2'-[2-(1,3-benzodioxol-5-yl)pyrimidin-4-yl]-5',6'-dihydrospiro[piperidine-4,7'-pyrrolo[3,2-c]pyridin]-4'(1'H)-one 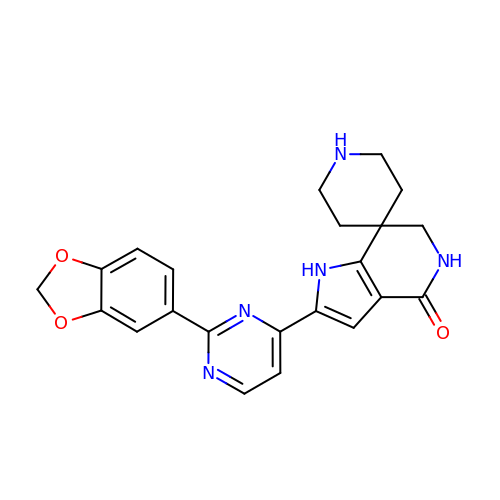| C22 H21 N5 O3 | QSDGMDKMSSYMKU-UHFFFAOYSA-N>GSADLAHGGQVFSANCAACHLGGRNVVNPAKTLQKADLDQYGMASIEAITTQVTNGKGAMPAFGSKLSADDIADVASYVLDQSEKGWQG[4x]

Cyt c6 is a small, water-soluble protein (~12 kDa) that contains a heme group as its active center. As an essential electron carrier, Cyt c6 mediates between the cytochrome b6f complex and photosystem I (PSI), enabling electron transfer that is fundamental for sustaining photosynthesis by maintaining the continuous flow of electrons through the photosynthetic chain. The crystal structures of Cyt c6 from both species revealed a conserved fold, consisting of five α-helices, a bound heme group, and loop regions, which closely resembled previously characterized Cyt c6 proteins from other species. The heme was covalently linked to two cysteine residues via thioether bonds, and the central iron atom was axially coordinated by methionine and histidine residues, maintaining consistent coordination geometry in both oxidized and reduced states.

Upon extracting and aligning these dimers, their positions were nearly identical, with a RMSD of 0.259 Å between the two distinct dimers in the Cyt c6-7942 tetramer. The results indicated that the red-Cyt c6-7942 forms a stable dimer. The dimerization is energetically favorable, with an interaction free energy of −54.6 kcal/mol. However, the dissociation energy of 0.7 kcal/mol implies that the dimer is weakly stable and may dissociate in specific conditions. Specifically, the key residues involved included Ala16, Val24, Val25, Gly56, Ala57, Met58, Pro59 and Lys64 for Cyt c6-7942. Structural comparisons between red-Cyt c6-7942 and oxi-Cyt c6-7942 revealed some differences in surface amino acids, particularly charged residues, despite the largely similar positions of heme-binding pocket residues. In red-Cyt c6-7942, Asp69 formed additional hydrogen bonds with His5, stabilizing the connection between two α-helices. Additionally, the hydrogen bond between Asn23 and Asn26, along with the interaction between Thr30 and Gln32, result in a more compact structure. In the reduced form, non-heme-binding sites contribute to a more compact structure, which helps stabilize the dimeric configuration. Small structural differences between red-Cyt c6-7942 and oxi-Cyt c6-7942 suggest insights into the functional mechanism of photosynthetic electron transfer.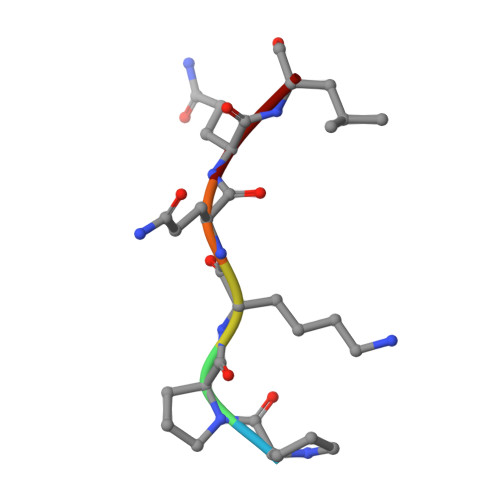> PPKQQL6-aminopyridine-3-carboxamide | 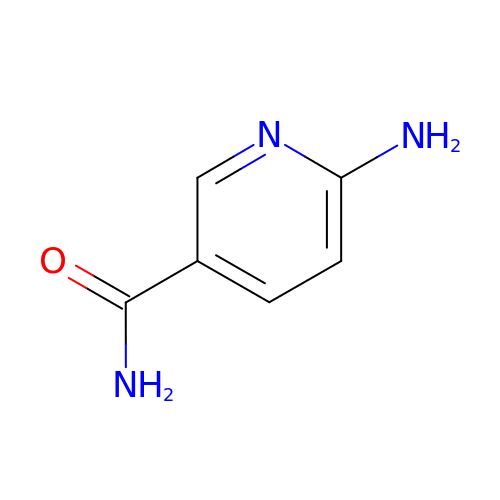C6 H7 N3 O | ZLWYEPMDOUQDBW-UHFFFAOYSA-N>GFARLKRSLLKTKENLGSGFISLFRGKKIDDDLFEELEEQLLIADVGVETTRKIITNLTEGASRKQLRDAEALYGLLKEEMGEILAKVDEPLNVEGKAPFVILMVGVNGVGKTTTIGKLARQFEQQGKSVMLAAGDTFRAAAVEQLQVWGQRNNIPVIAQHTGADSASVIFDAIQAAKARNIDVLIADTAGRLQNKSHLMEELKKIVRVMKKLDVEAPHEVMLTIDASTGQNAVSQAKLFHEAVGLTGITLTKLDGTAKGGV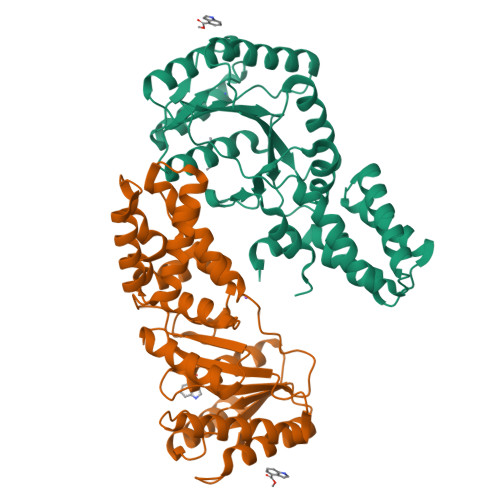IFSVADQFGIPIRYIGVGERIEDLRPFKADDFIEALFARED[2x]(3R,4S)-3-(3-carboxyphenyl)-4-propyl-L-proline 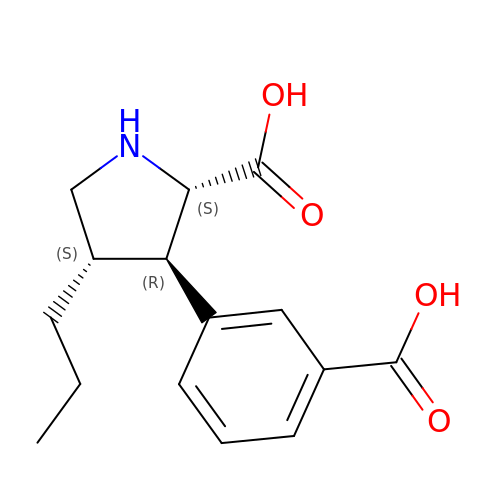| C15 H19 N O4 | OORLOXOWCACWSS-AGIUHOORSA-N> MAAIDKLVKASHLIDMNDIIREGNPTLRKVAEEVTFPLSEKEEIL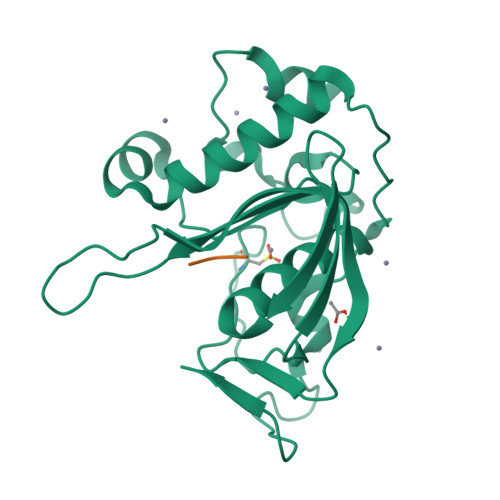GEKMMQFLKHSQDPIMAEKLGLRGGVGLAAPQLDISKRIIAVLVPNVEDAQGNPPKEAYSLQEVMYNPKVVSHSVQDAALSDGEGCLSVDREVPGYVVRHARVTIEYFDKTGEKHRLKLKGYNSIVVQHEIDHIDGIMFYDRINEKNPFAVKEGLLILE;> MAS methyl 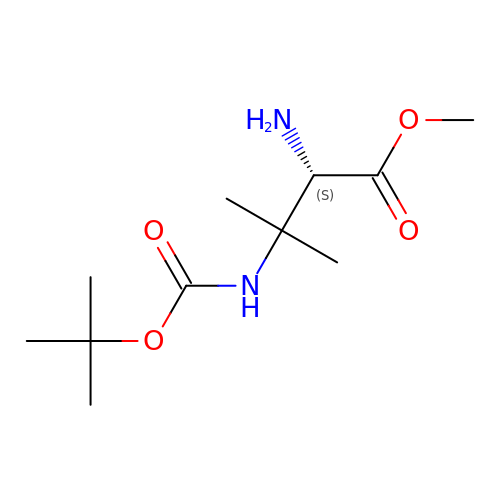(2S)-2-azanyl-3-methyl-3-[(2-methylpropan-2-yl)oxycarbonylamino]butanoate | C11 H22 N2 O4 | UTWVEOUYCGZORL-SSDOTTSWSA-N7-(5-bromo-2-ethoxyphenyl)-6-methylquinazoline-2,4-diamine 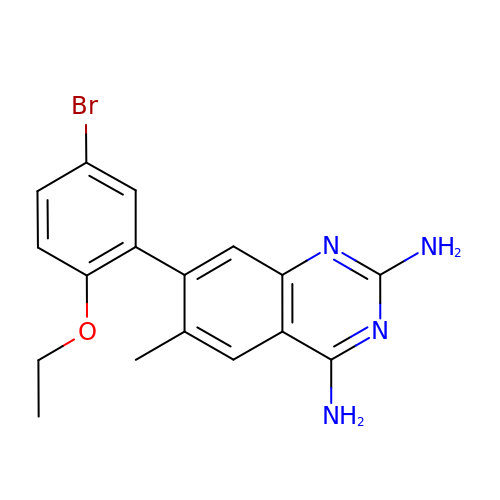| C17 H17 Br N4 O | YCEDXTDKSNASDG-UHFFFAOYSA-N Here, we present a new pipeline, SIMBAD (Sequence-Independent Molecular replacement Based on Available Databases), which can be used for both contaminant and brute-force approaches. In this section, we present three cases in which SIMBAD has been used to determine a difficult-to-solve case owing to the unwitting crystallization of a contaminant. All cases involve the crystallization of a known contaminant. Although the targets were ultimately of low importance for the structural insights that they provided, their solution prevented further misdirected effort on the part of the researchers involved.

Crystals of the contaminant protein (cyanase) grew in conditions expected to crystallize a cytokine complex: the vapour-diffusion method with a well solution consisting of 0.1 M magnesium acetate, 10% PEG 10K, 0.1 M MES pH 6.5 and hanging drops composed of a 1:1 mixture of the well solution and the protein complex. Crystals appeared after six months at ambient temperature. The crystals were cryoprotected with 20% ethylene glycol. The crystals belonged to space group C121, with lattice parameters a = 136.56, b = 94.13, c = 89.11 Å, α = 90, β = 125.49, γ = 90° and five molecules in the asymmetric unit. After refinement it became clear that this was the protein that had crystallized instead of the cytokine complex. Manual model inspection and modifications were performed with Coot. In the crystal, ten molecules of the protein form a dimeric pentagonal ring. Normally, this is a logical step that saves computing time; however, this case demonstrates the value of making no assumptions where contaminant origin is concerned. SIMBAD has subsequently been modified as a result of this case to use a Matthews coefficient to check whether a search model can fit into the asymmetric unit prior to MR. If the full PDB entry is too large to be used as a search model, only the first chain is used. This alteration allowed a solution to be found at the lattice-parameter search instead of the MoRDa DB search in subsequent testing.

>MTQSLHYSSPRETLTDTIMMAKIRKNLTFEAINQGTGLSLAFVTAALLGQHPLPEQAARVVAEKLDLDEDAIRLLQTIPLRGSIPGGVPTDPTIYRFYEMVQIYGSTLKALVHEQFGDGIISAINFKLDIKKVPDPDGGERAVITLDGKYLPTKPF[5x]5'-O-[(R)-(2-amino-1H-imidazol-1-yl)(sulfanyl)phosphoryl]guanosine 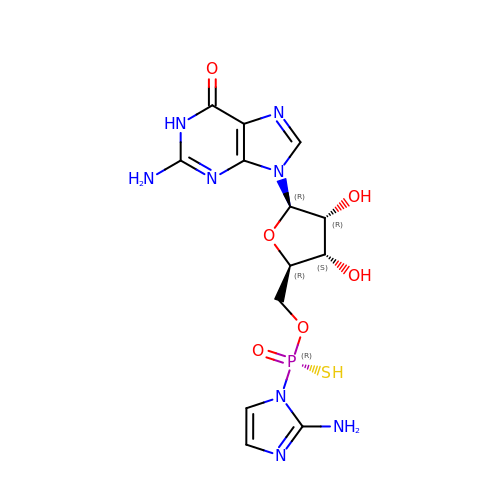| C13 H17 N8 O6 P S | KURJQYGWAXZKPO-RMPAVHDKSA-N> MSLEWQDLAQLP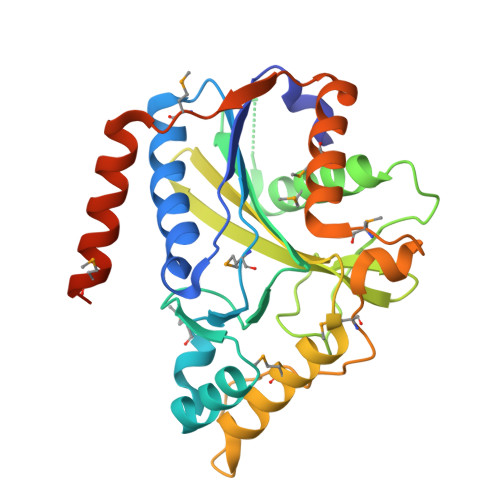VSIFKDYVTDAQDAEKPFIWTEVFLREINRSNQEIILHIWPMTKTVILGMLDRELPHLELAKKEIISRGYEPVVRNFGGLAVVADEGILNFSLVIPDVFERKLSISDGYLIMVDFIRSIFSDFYQPIEHFEVETSYCPGKFDLSINGKKFAGLAQRRIKNGIAVSIYLSVCGDQKGRSQMISDFYKIGLGDTGSPIAYPNVDPEIMANLSDLLDCPMTVEDVIDRMLISLKQVGFNDRLLMIRPDLVAEFDRFQAKSMANKGMVSRDEEGHHHHHH>MDFLSNFLTDFVGQLQSPTLAFLIGGMVIAALGTQLVIPEAISTIIVFMLLTKIGLTGGMAIRNSNLTEMLLPVAFSVILGILIVFIARFTLAKLPNVRTVDALATGGLFGAVSGSTMAAALTTLEESKISYEAWAGALYPFMDIPALVTAIVVANIYLNKRKRKSAAASIEESFSKQPVAAGDYGDQTDYPRTRQEYLSQQEPEDNRVKIWPIIEESLQGPALSAMLLGLALGIFTKPESVYEGFYDPLFRGLLSILMLIMGMEAWSRIGELRKVAQWYVVYSLIAPIVHGFIAFGLGMIAHYATGFSLGGVVVLAVIAASSSDISGPPTLRAGIPSANPSAYIGSSTAIGTPIAIGVCIPLFIGLAQTLGAG[3x]

SbtA, which is ubiquitous in cyanobacteria, is an inducible high-affinity sodium-dependent HCO3– symporter within the TC.2.A.83 family of Na+/solute symporters. The sbtB gene from the sbtA–sbtB operon encodes a PII-like signaling protein that senses the intracellular level of the secondary messenger cAMP that correlates with high Ci conditions, versus AMP at low Ci conditions, thus functioning as a Ci sensor in cyanobacteria. The tightly packed trimeric structure of SbtA is exclusively stabilized by the gate domains at the center, with a threefold axis perpendicular to the membrane plane. In summary, this study provides structural insights into the cyanobacterial high-affinity HCO3– transporter SbtA, which exhibits a new architecture of Na+/solute symporters and its fine interaction pattern with a PII-like protein SbtB.

Here we purified Synechocystis sp. PCC 6803 SbtA and solved its cryo-EM structure at 3.50 Å resolution. Notably, the TM4 and TM9 helices in the core domain are unfolded and form a crossover at the middle. In the gate domain, TM1 and TM6 are divided into two helical moieties, forming a kink at the middle. Structural analysis showed that SbtA of a 5 + 5 fold is topologically similar to Neisseria meningitides ASBT8. The trefoil-like helical bundle of the gate domains possesses a completely buried interface area of ~3000 Å2, mainly via hydrophobic interactions. Structural analysis revealed that the substrate-binding sites of free SbtA are inaccessible to the solvent from either intracellular or extracellular side. Thus, the structure of free SbtA represents an occluded conformation. Substrate binding most likely promotes SbtA to adopt an occluded conformation, as seen in our free SbtA structure with a Na+ bound in the pocket.> MSIDWEQTFRKWSKPSSETESTKAENAERMIKAAINSSQILSTKDISVFPQGSYRNNTNVREDSDVDICVCLNTLVLSDYSLVPGMNDKLAELRTASYTYKQFKSDLETALKNKFGTLGVSRGDKAFDVHANSYRVDADVVPAIQGRLYYDKNHNAFIRGTCIKPDSGGTIYNWPEQNYSNGVNKNKSTGNRFKLIVRAIKRLRNHLAEKGYNTAKPIPSYLMECLVYIVPDQYFTGDSYKTNVENCINYLYNQIDSSDWTEINEIKYLFGSHQMWNKTQVKEFLLTAWSYIQKNLEHHHHHH

Here, we determine the high-resolution structures of cyclic di-pyrimidine-synthesizing cGAS/DncV-like nucleotidyltransferases (CD-NTases) in clade E (CdnE) in its apo, substrate-, and intermediate-bound states. CD-NTases share an N-terminal core domain with templated and non-templated polymerases of the nucleotidyltransferase (NTase) superfamily, but the C-terminal helical domain shows a higher degree of variation. Three conserved acidic residues in the central β-sheet of the NTase domain coordinate with two metal ions (A and B) that are essential for catalysis. Based on sequence conservation and structural similarity, it is proposed that the cyclic di-pyrimidine-synthesizing CdnE proteins, including ClCdnE, EfCdnE, and LpCdnE, form smaller donor pockets that act as molecular gauges to recognize and retain the binding of pyrimidine nucleotides but weaken or exclude the binding to purine nucleotides.

The native structure of LpCdnE was refined to 2.46-Å resolution. It differs from ClCdnE in similar regions, with 1.32 Å RMSD for 276 Cα pairs, but the α1-α2 loop is missing. LpCdnE, which makes cUU, shows 36% and 34% sequence identity to ClCdnE and EfCdnE, respectively, which is slightly higher than the 32% and 31% identity to EmCdnE and RmCdnE, respectively. Despite the differences in local regions, the dispositions of the NTase and helical domains were similar in the native structures of ClCdnE, EfCdnE, and LpCdnE, respectively. The four protein models, two from LpCdnE-UTP and two from LpCdnE-UMPnPP complex show RMSD of 0.56 Å to 0.82 Å from the native LpCdnE for 281 to 286 matched Cα pairs.> MHHHHHHGGGENLYFQGTAGLGYGSWEIDPKDLTFLKELGTGQFGVVKYGKWRGQYDVAIKMIKEGSMSEDEFIEEAKVMMNLSHEKLVQLYGVCTKQRPIFIITEYMANGCLLNYLREMRHRFQTQQLLEMCKDVCEAMEYLESKQFLHRDLAARNCLVNDQGVVKVSDFGLSRYVLDDEYTSSVGSKFPVRWSPPEVLMYSKFSSKSDI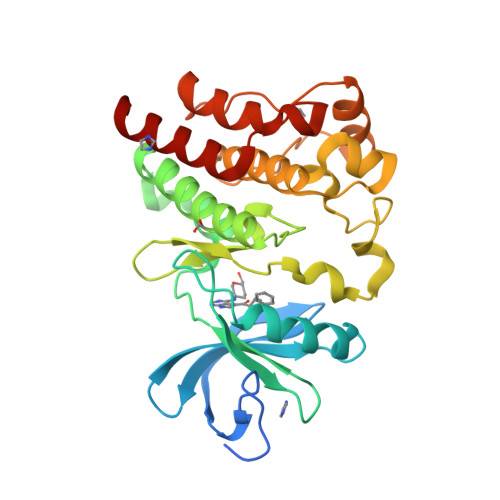WAFGVLMWEIYSLGKMPYERFTNSETAEHIAQGLRLYRPHLASEKVYTIMYSCWHEKADERPTFKILLSNILDVMDEES> XIGRRLPPTP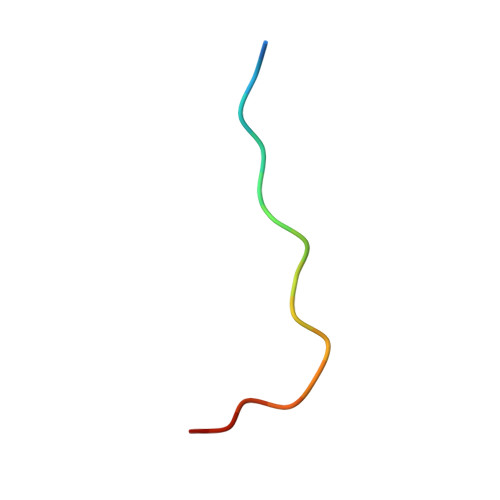SKPSTLX PLK4, the master regulator of centriole duplication, is the most distant member of the family. It is distinguished from all other PLKs by the presence of a third C-terminally located Polo-box, PB3, in addition to the two central and closely linked Polo-boxes PB1 and PB2. Here, we demonstrate that monomeric PB3 of human PLK4 adopts a canonical Polo-box-fold and directly interacts with nanomolar affinity with the central STIL-CC region, STIL-CC. Most importantly, we determined the solution structure of the human PLK4-PB3 and a crystal structure of the PLK4-PB3/STIL-CC complex and use structure-based mutagenesis of STIL to demonstrate an essential role of STIL-CC for PLK4 binding and the regulation of centriole biogenesis in vivo.

In contrast, plate-like crystals of the PLK4-PB3/STIL-CC complex diffracting to 2.6 Å resolution were obtained using seeding. The structure was solved by molecular replacement, and refined to Rwork/free of 0.22/0.25, respectively with one monomeric PLK4-PB3/STIL-CC per asymmetric unit. The NMR structure of PLK4-PB3 in solution and the crystal structure of its STIL-CC complex display a conserved overall fold comprising a six-stranded antiparallel β-sheet (β1–β6) and a C-terminal α-helix (α1), which packs against the β-sheet and contacts residues from all six strands. PLK4-PB3 and STIL-CC interact along the entire STIL-helix and form a substantial interface of 934 Å2 buried surface area. Two regions on PLK4-PB3 contribute to the predominantly hydrophobic binding interface: First, the surface of the PLK4-PB3 β-sheet around residues V907, L917, V919, I926 and Y928, and second the α1 helix (I948, L952, L955 and L959) and the linker (L944) leading into it. Key interacting residues on STIL-CC are leucine and isoleucine residues (L733, L736, I740, L743, L744) pointing towards the hydrophobic surface of PLK4-PB3. Additional interactions are provided by backbone–backbone hydrogen bonds between PB3G922-STILQ739 and PB3K943-STILM750, respectively. PLK4-PB3 reveals a novel binding mode by interacting with the helical STIL-CC region in a leucine-zipper-style via the α1 helix with further hydrophobic contacts to the central β-sheet. Overall, the structural data reveal two core differences in PLK4-PB3 induced by STIL-CC binding: first, strand β1 is N-terminally extended by three residues to the range 888–893, resulting in a shortening of the unstructured N-terminal region in the STIL-CC complex. Second, helix α1 slightly changes its orientation and is stabilized by STIL-CC binding.

> SAQLLKSVFVKNVGWATQLTSGAVWVQFNDGSQLVVQAGVSSISYTSPNGQTTRYGENEKLPDYIKQKLQCLSSILLMFSNPTPNFH;> PDAYRFLTEQDRQLRLLQAQIQRLLEAQSLMP> MNNNKAEADTSSSMADPETRPTYTTHHLAIPSGVTQDEFDELKQSVVEFHTYQLSQNQCSSLLAQRIRAPNDVVWSIVRRFDQPQTYKHFIKSCSVSDNFTMAVGSTRDVNLISGLPAATSTERLDILDDDRQVLGISIIGGEHRLRNYRSVISVHGFNRDGAICTVALESYVVDVPEGNTEEDTRLFADTVVK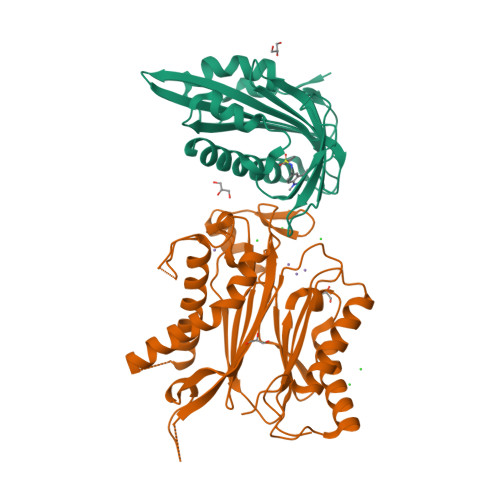LNLQKLVSVAESQVI;> RSVYELDCIPLWGVVSIQGNRSEMEDAFAVSPHFLKLPIKMLMGDHEGMSPSLTHLTGHFFGVYDGHGGHKVADYCRDRLHFALAEEIERIKDELCKRNTGEGRQVQWDKVFTSCFLTVDGEIEGKIGRAVVGSSDKVLEAVASETVGSTAVVALVCSSHIVVSNCGDSRAVLFRGKEAMPLSVDHKPDREDEYARIENAGGKVIQWQGARVFGVLAMSRSIGDRYLKPYVIPEPEVTFMPRSREDECLILASDGLWDVMNNQEVCEIARRRILMWHKKNGAPPLAERGKGIDPACQAAADYLSMLALQKGSKDNISIIVIDLKAQRKFKTRT> MSLDKVLVGYWHNWKSTGKDGYKGGSSADFNLSSTQEGYNVINVSFMKTPEGQTLPTFKPYNKTDTEFRAEISKLNAEGKSVLIALGGADAHIELKKSQESDFVNEIIRLVDTYGFDGLDIDLEQAAIEAADNQTVIPSALKKVKDHYRKDGKNFMITMAPEFPYLTSSGKYAPYINNLDSYYDFINPQYYNQGGDGFWDSDLNMWISQSNDEKKEDFLYGLTQRLVTGTDGFIKIPASKFVIGLPSNNDAAATGYVKDPNAVKNAL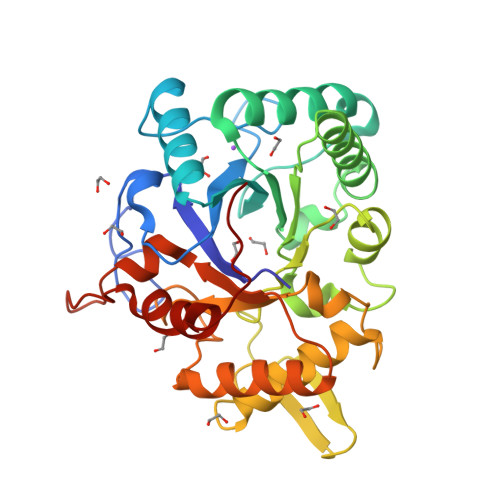NRLKASGNEIKGLMTWSVNWDAGTNSNGEKYNNTFVNTYAPMLFNNEGHHHHHH[[[(2~{R},3~{R},4~{R},5~{R})-5-(2-azanyl-7-methyl-6-oxidanyl-purin-7-ium-9-yl)-4-methoxy-3-oxidanyl-oxolan-2-yl]methoxy-oxidanyl-phosphoryl]oxy-selanyl-phosphoryl] 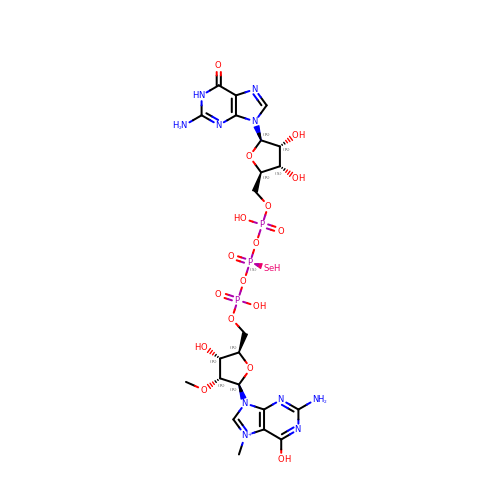[(2~{R},3~{S},4~{R})-5-(2-azanyl-6-oxidanylidene-1~{H}-purin-9-yl)-3,4-bis(oxidanyl)oxolan-2-yl]methyl hydrogen phosphate | C22 H32 N10 O17 P3 Se | LVNVABJMRYMPGM-DCILJVRDSA-O> KNIINTSILNLRYESNHLIDLSRYASKINIGSKVNFDPIDKNQIQLFNLESSKIEVILKNAIVYNSMYENFSTSFWIRIPKYFNSISLNNEYTIINCMENNSGWKVSLNYGEIIWTLQDTQEIKQRVVFKYSQMINISDYINRWIFVTITNNRLNNSKIYINGRLIDQKPISNLGNIHASNNIMFKLDGCRDTHRYIWIKYFNLFDKELNEKEIKDLYDNQSNSGILKDFWGDYLQYDKPYYMLNLYDPNKYVDVNNVGIRGYMYLKGPRGSVMTTNIYLNSSLYRGTK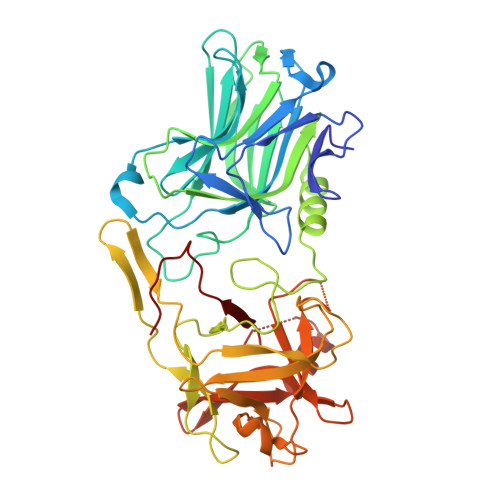FIIKKYASGNKDNIVRNNDRVYINVVVKNKEYRLATNASQAGVEKILSALEIPDVGNLSQVVVMKSKNDQGITNKCKMNLQDNNGNDIGFIGFHQFNNIAKLVASNWYNRQIERSSRTLGCSWEFIPVDDGWGERPL>[2x]MTLEKFVDALPIPDTLKPVQQSKEKTYYEVTMEECTHQLHRDLPPTRLWGYNGLFPGPTIEVKRNENVYVKWMNNLPSTHFLPIDHTIHHSDSQHEEPEVKTVVHLHGGVTPDDSDGYPEAWFSKDFEQTGPYFKREVYHYPNQQRGAILWYHDHAMALTRLNVYAGLVGAYIIHDPKEKRLKLPSDEYDVPLLITDRTINEDGSLFYPSAPENPSPSLPNPSIVPAFCGETILVNGKVWPYLEVEPRKYRFRVINASNTRTYNLSLDNGGDFIQIGSDGGLLPRSVKLNSFSLAPAERYDIIIDFTAYEGESIILANSAGCGGDVNPETDANIMQFRVTKPLAQKDESRKPKYLASYPSVQHERIQNIRTLKLAGTQDEYGRPVLLLNNKRWHDPVTETPKVGTTEIWSIIN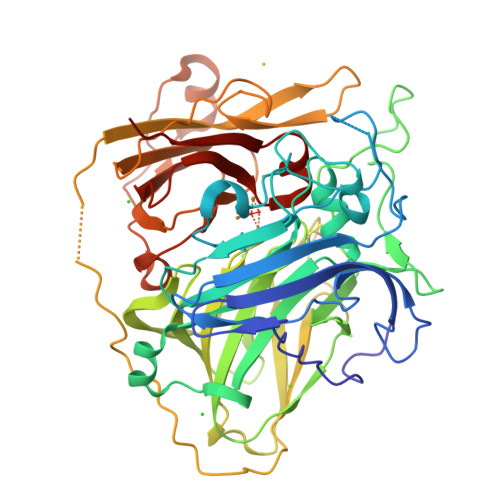PTRGTHPIHLHLVSFRVLDRRPFDIARYQESGELSYTGPAVPPPPSEKGWKDTIQAHAGEVLRIAATFGPYSGRYVWHCHILEHEDYDMMRPMDITDPHK>ETGSAQQLNEDLRLHLLLNTSVTCNDGSPAGYYLKESRGSRRWLLFLEGGWYCFNRENCDSRYDTMRRLMSSRDWPRTRTGTGILSSQPEENPYWWNANMVFIPYCSSDVWSGASSKSEKNEYAFMGALIIQEVVREL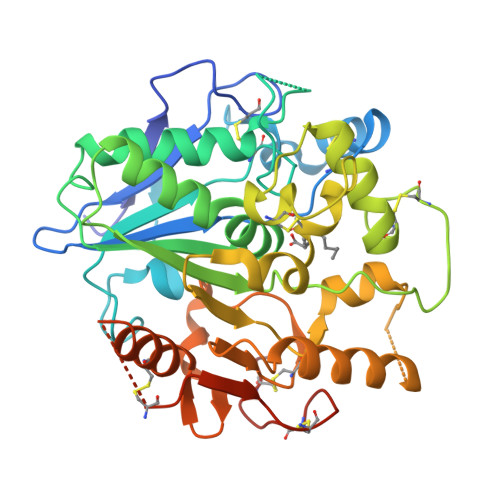LGRGLSGAKVLLLAGSAAGGTGVLLNVDRVAEQLEKLGYPAIQVRGLADSGWFLDNKQYRHTDCVDTITCAPTEAIRRGIRYWNGVVPERCRRQFQEGEEWNCFFGYKVYPTLRSPVFVVQWLFDEAQLTVDNVHLTGQPVQEGLRLYIQNLGRELRHTLKDVPASFAPACLSHEIIIRSHWTDVQVKGTSLPRALHCWDRSLHDSHKASKTPLKGCPVHLVDSCPWPHCNPSCPTGTHHHHHHHHHH[2x]>[3x]GAMKNEYLLLTPGPLSTSEAVREAMLKDWCTWDDEYNKD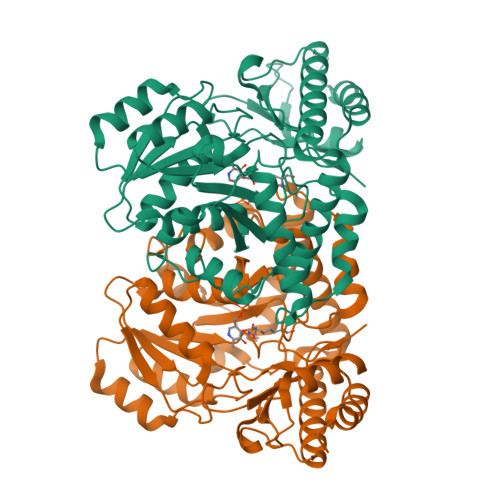IVEVIRTKLVKLATKHSGYTSVLMQGSGTASVEATIGSAIGKEGKLLVVDNGAYGARIAQIADYLNIPCHAVSPGETSQPHLNEVETALASDPAITHVAIVHCETTTGMLNPIEAFASAAKAHGKVVILDAMSSFGGIPIDIAELGIDFMISSANKCIQGVPGFGFVIAKKTELEKCQGQARSLSLDLYDQWHCMEVNHGKWRFTSPTHTVRAFYQALLELEQEGGIEARHNRYQTNQKTLVAGMRSLGFEPLLSDDLHSPIITSFYSPTHSDYQFKAFYTRLKEQGFVIYPGKVSNADCFRIGNIGEVYPADIERLIGAIEKAMYWQVA> MRSKFKDEHPFEKRKAEAERIRQKYTDRIPVICEKVEKSDIATIDKKKYLVPADLTVGQFVYVIRKRIKLSPEKAIFIFVQDTLPPTAALMSSIYELHKDEDGFLYITYSGENTFGDLFEE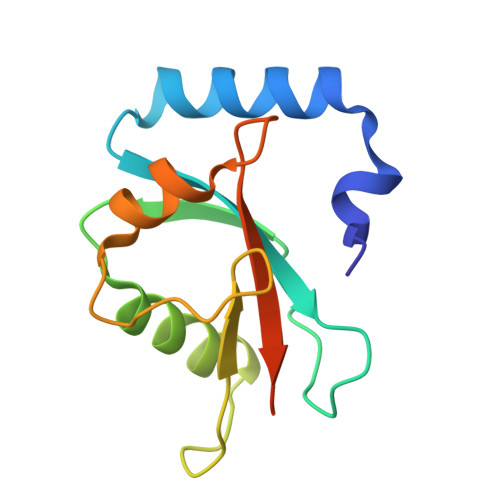VE>LPRETDEEPEEPGRRGSFVEMVDNLRGKSGQGYYVEMTVGSPPQTLNILVDTGSSNFAVGAAPHPFLHRYYQRQLSSTYRDLRKGVYVPYTQGKWE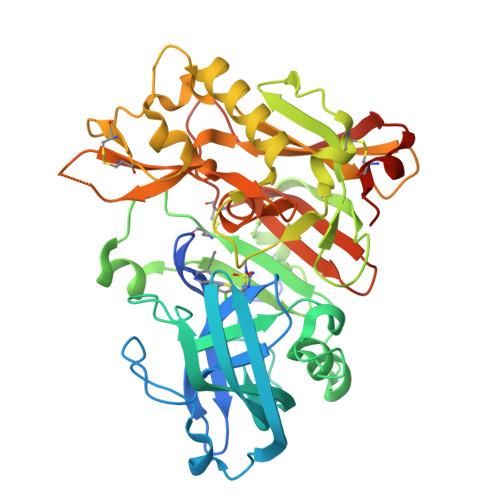GELGTDLVSIPHGPNVTVRANIAAITESDKFFINGSNWEGILGLAYAEIARPDDSLEPFFDSLVKQTHVPNLFSLQLCGAGFPLNQSEVLASVGGSMIIGGIDHSLYTGSLWYTPIRREWYYEVIIVRVEINGQDLKMDCKEYNYDKSIVDSGTTNLRLPKKVFEAAVKSIKAASSTEKFPDGFWLGEQLVCWQAGTTPWNIFPVISLYLMGEVTNQSFRITILPQQYLRPVEDVATSQDDCYKFAISQSSTGTVMGAVIMEGFYVVFDRARKRIGFAVSACHVHDEFRTAAVEGPFVTLDMEDCGYNIPQTDEST[2x]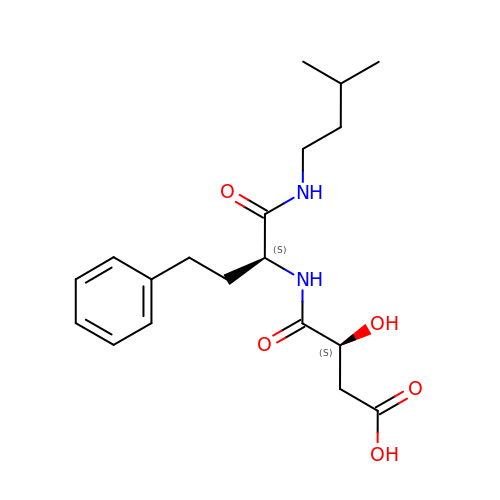N-[3-CARBOXY-2-HYDROXY-PROPIONYL]-L-HOMOPHENYLALANYL-AMINO-2-METHYLBUTANE | C19 H28 N2 O5 | KVZMXOVSHIMGNA-HOTGVXAUSA-N> GSHMHESKEWYHASLTRAQAEHMLMRVPRDGAFLVRKRNEPNSYAISFRAEGKI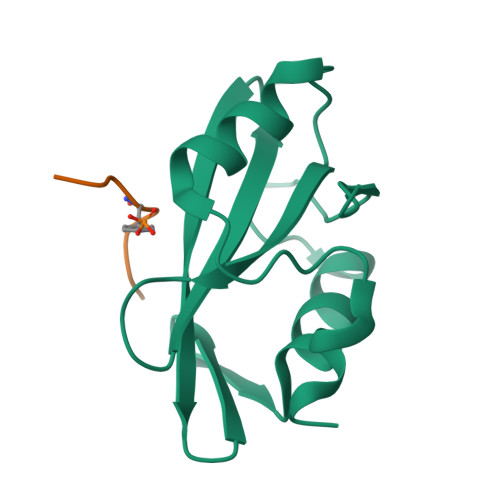KHCRVQQEGQTVMLGNSEFDSLVDLISYYEKHPLYRKMKLRYPINEE;> PSSVYVPDEWE> KSGKPSGEMDEVGVQKCKNALKLPVLEVLPGGGWDNLRNVDMGRVMELTYSNCRTTEDGQYIIPDEIFTIPQKQSNLEMNSEILESWANYQSSTSYSINTELSLFSKVNGKFSTEFQRMKTLQVKDQAITTRVQVRNLVYTVKINPTLELSSGFRKELLDISDRLENNQTRMATYLAELLVLNYGTHVTTSVDAGAALIQEDHLRASFLQDSQSSRSAVTASAGLAFQNTVNFKFEENYTSQNVLTKSYLSNRTNSRVQSIGGVPFYPGITLQAWQQGITNHLVAIDRSGLPLHFFINPNMLPDLPGPLVKKVSKTVETAVKRYYTFNTYPGCTDLNSPNFNFQANTDDGSCEGKMTNFSFGGVYQECTQLSGNRDVLLCQKLEQKNPLTGDFSCPSGYSPVHLLSQIHEEGYNHLECHRKCTLKVFCKTVCEDVFQVAKAEFRAFWCVASSQVPENSGLLFGGLFSSKSINPMTNAQSCPAGYFPLRLFENLKVCVSQDYELGSRFAVPFGGFFSCTVGNPLVDPAISRDLGAPSLKKCPGGFSQHPALISDGCQVSYCVKSGLFTGGSLPPARLPPFTRPPLMSQAATNTVIVTNSENARSWIKDSQTHQWRLGEPIELRRAMNVIHGDGGGLSHHHHHH

Macrophage-expressed gene 1 (MPEG1, also termed Perforin-2) is one of the most ancient and highly conserved members of the membrane attack complex (MAC)/perforin-like (PF)/cholesterol-dependent cytolysin (MACPF/CDC) superfamily, with orthologous sequences identifiable throughout the metazoan. In contrast to other perforin-like proteins characterised to date, human MPEG1 is an integral type-1 transmembrane protein. The mature protein is comprised of three regions; an ectodomain located in the vesicular lumen, a transmembrane domain anchor that spans the vesicular membrane and, finally, a short cytosolic sequence. Each monomer of the 16-subunit ring possesses an N-terminal MACPF/CDC domain, a central multi-vesicular body of 12 kDa (MVB12)-associated β-prism (MABP) domain and a C-terminal region (termed the L-domain).

Indeed, our (ultimately unsuccessful) attempts to disrupt the interface between the double ring serendipitously led to our identifying the MPEG1 L425K mutation as yielding a greatly improved sample and an improvement in global resolution to 2.4 Å (workflow described in detail in the methods). This mutation resulted in two different MPEG1L425K assemblies, one of which involved domain swapping between the two head-to-head coordinated rings. In contrast, the MPEG1 MABP domain possesses <5% primary amino-acid sequence similarity to other homologues and the fold was accordingly identified using Dali searches. The L-domain directly precedes the transmembrane region and includes a short two-stranded β-sheet capped by an α-helix. Within each subunit, both TMH-1 and -2 are folded as small helical bundles. The L-domain forms substantial inter-subunit interactions in trans with an extraordinary elongated β-hairpin that extends from the MABP domain of the adjacent subunit (the MABP β-hairpin).>[2x]MAETRVIVVGNEKGGAGKSTIAVHLVTALLYGGAKVAVIDLALRQRTSARFFENRRAWLDNKKIELPEPLALNLSDNDVALAERPEEEQVAGFEAAFARAMAECDFILIDTPGGDSAITRMAHGRADLVVTPMNDSFVDFDMLGTVDPVTLELTKPSLYSLTVWEGRKQRALS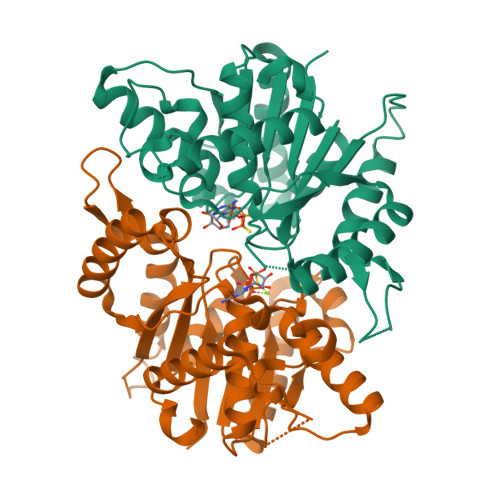GQRQAMDWVVLRNRLATTEARNRKRLEDRLNALAKRVGFRIGPGLRDRVIYRELFPFGLTIADLSPQVRPVPVSLQHLAARQELRALMHSLGLSAYSGETMLAAQGSHHHHHH Cyanobacteria, glaucophytes, and rhodophytes utilize a large water-soluble, light-harvesting complex called phycobilisome (PBS) for solar energy absorption and energy transfer to photosynthetic membrane proteins (photosystem I and photosystem II; PSI and PSII). PBS is composed of phycobiliproteins (PBPs) such as phycoerythrin, phycoerythrocyanin, phycocyanin (PC), and allophycocyanin (APC). Oligomers of these α- and β-subunits interact with non-chromophorylated linker proteins to form PC rods in the whole PBS complex. Here, we report the structures of the pentacylindrical APC core and PC rod from the thermophilic cyanobacterium Thermosynechococcus vulcanus at the resolutions of 3.7 Å and 4.2 Å, respectively.

The analyzed PBS core of T. vulcanus shows a hemidiscoidal structure with C2 symmetry, composed of three cylinders (A, A’, and B), two cylinders (C and C’) with some PC rods interacting with the PBS core. The PBS core is a supercomplex with the dimensions 110 × 210 × 300 Å and is composed of 38 ApcAs, 40 ApcBs, 6 ApcCs, 2 ApcDs, 2 ApcEs (LCMs), 2 ApcFs, and 84 PCBs. In the other cyanobacterial PBS core, the A and B cylinders each consist of four APC trimers, whereas the PBS core of T. vulcanus comprises three APC trimers in the A cylinder and four APC trimers in the B cylinder. The A (A’) cylinder consists of three APC trimers (A1, A2, and A3) with subunits of ApcD/ApcB and two ApcA/ApcB (A1); three ApcA/ApcB (A2); and ApcE/ApcB, ApcA/ApcF, and ApcA/ApcB (A3), respectively. ApcE (LCM) is a terminal emitter that is located at the membrane surface in the A cylinder and transfers energy to PSII. ApcE (LCM) consists of αLCM, and one of its domains exhibits a similar structure to ApcA, four repeated motifs named “repeats” (Rep1–Rep4), and “arms” (Arm1–3) that connect the motifs. The energy transfer from the C (C’) cylinder to the B and A (A’) cylinders occurs via C1α184–B1α284 (33 Å) and C2α384–A2α384 (35 Å), respectively. Three PCBs in the A cylinder (A2α384, A2α284, and A3α384) are believed to be the key chromophores that receive excitation energy from the B and C cylinders based on their spatial arrangement, which then ultimately pass it to the chromophore (A3αLCM198) in the terminal emitters. In the T. vulcanus PBS, the distance between A3βApcF82 and A3αLCM198 is 20 Å, suggesting that the two chromophores could form an excitonic coupling that eventually transfers excitation energy to PSI and PSII. Nevertheless, the present structure suggests that A3αLCM198 in ApcE could form a π–π interaction with W166/AcpE, as the D-ring of PCB and tyrosine residues in ApcA commonly form a π–π interaction.

>[40x]MSVVTKSIVNADAEARYLSPGELDRIKNFVSTGERRLRIAQTLTENRERIVKQAGDQLFQKRPDVVSPGGNAYGEEMTATCLRDLDYYLRLVTYGIVAGDVTPIEEIGLVGVREMYNSLGTPIPAVAEGIRAMKNVACSLLSAEDAAEAGSYFDFVIGAMQ;>MQDAITAVINASDVQGKYLDTAAMEKLKAYFATGELRVRAASVISANAANIVKEAVAKSLLYSDITRPGGNMYTTRRYAACIRDLDYYLRYATYAMLAGDPSILDERVLNGLKETYNSLGVPIAATVQAIQAMKEVTASLVGADAGKEMGIYFDYICSGLS[40x];>MVVKASGGSSVARPQLYQTVPVSTIIQAEQQDRFLNRGELDELAVYLRSGAKRLEIATTLTRNADIIVSRAANRIFVGGSPMAFLSRPQTEEAPQFTTGARGEAIDIKEAMKLGTATYVDTRGGFLEGLRSIFSASSGGAPVGFKPINIARYGPARMEKSLRDLDWFLRYTTYAIVAGDPNILAVNTRGLREIIEAACSSDATIAALQEMRRAALSYFEKDAEAKGIVETYFDVLINEFIAPAPSDKVRQRNSTDLQGLQLPQIYFNAAERRPKFVMKPGLSAAEKNEVVKAAYRQIFERDISRAYGLGISDLESKVKNGSISMKEFIRQLAKSPLYRKNFYEPYINSRALELAFRHILGRGPSSREEVQTYFAIISKGGLPALVDALVDSKEYSDYFGEETVPYLRGLGQEAQECRNWGAQQDLFKYSAPFRKVPQFITTFAAQDQPLPDQHPYGSGNDPLEIQFGAIFPKEKKNPSARPQPFNKDTRRILIARGPGINNQVSNPGARGLTPGTLGPKVFKLDQLPSINARIGKRSIATGTDSVKFAESSTQRVIRAAYLQVFGRDVYEGQRQKVAEIKLENGEISVREFVRILAKSNLFRSLYWTPLYVTKAIEYIHRRLLGRPTYGRQEMNAYFDIASKKGLYGLVDAIIDSQEYSEAFGEDTVPYERYITPQGLALRSLRVGTIGETGVPPEKEETPRFVELGAVTELRTEPAIQFRANQGVSKRREQTKVFKLTDLNDKQNLQLVIQAAYRQVFERDVAPYIVRDEFTALESKLSNGEITLKEFIEALGCSELYQKEFYTPYPNTKVIELGTKHFLGRAPLDQAEIRRYNQILATQGLKAFVQALVSSAEYAQAFGEDTVPYRRFPTLPAANFPNTEKLHNQLTKQSDAIVVPSFAPVKPRLDNTKLPLLSRAIAEQEAKARQADPSKPRFIELGRSFRNGDGQSVEVGVGTTRRRPARIFRMTVGAPSAEVELVINAIYCQVMDVFSGQVPSQFRRPDLESRLRNGEITVREFVRTLASSEIYRNRFYTPYPNTKVIEFLFRHLLGRAPATQAEIRQYNKILADQGLKTAVETMVNSPEYSRYFGEDVVPYKRFPTLPAGNYIGSVKADADLVKQSWSSLSPSLVGIQPSHRD[2x];>[2x]MRDAVTTLIKNYDSTGRYLDRDAVDRLRSYFNSGAARVKAAAVINANAAAIVKEAASALFTEQPELIQPGGNAYTTRRYATCLRDMDYYLRYASYAIVAGDVDVLNERVLEGLRETYNSLGVPIGPTVRGIQIMKEIVRDRVAAAGIEDTGIVEQPFDYMCRQLSEVNI;>[6x]MRMFKITACVPSQTRIRTQRELQNTYFTKLVPYENWFREQQRIQKMGGKIVKVELFTGKPGVNTGLA>[14x]MHRTYSLRNQRAPTAAELQAPPPPPSSTKSKFFGKASIASSFRKNAAGNFGPELARKLSQLVKTEKGVLRAMEVVASERREAAKQLSLWGADNDDDVSDVTDKLGVLIYELGELQDQFIDKYDQYRVTLKSIRNIEASVQPSRDRKEKITDEIAHLKYKDPQSTKIPVLEQELVRAEAESLVAEAQLSNITREKLKAAYSYMFDSLRELSEKFALIAGYGKALLELLDDSPVTPGEA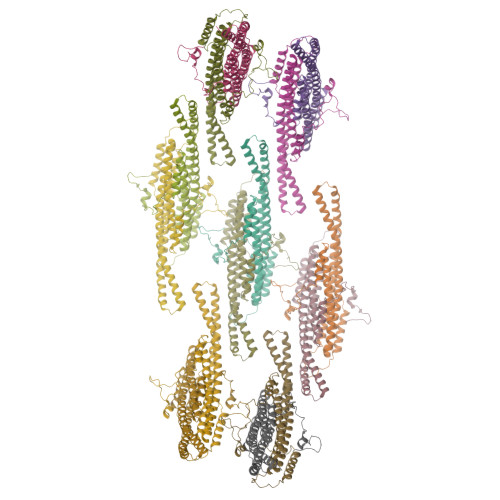RPAYDGYEASRQIIMDAESALESWTLDMAAVKPTLSFHQTVDDVYEDEDGEEEEEPEIQNGDIPGQVVEEEEVEWTTEVPVDDEAHEADHHVSQNGHTSGSENI>[2x]MPPGKCLFSGVF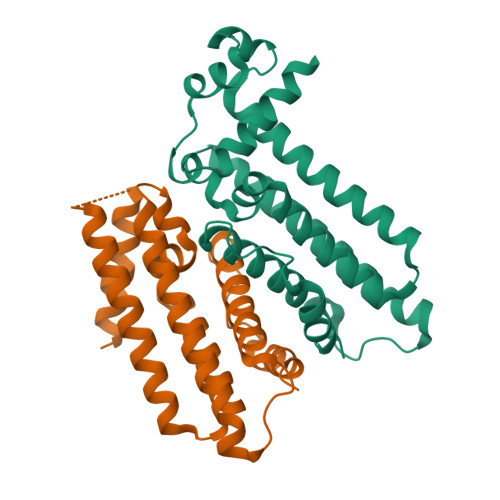CNMAEKQTAKRNRREEILQSLALMLESSDGSQRITTAKLAASVGVSEAALYRHFPSKTRMFDSLIEFIEDSLITRINLILKDEKDTTARLRLIVLLILGFGERNPGLTRILTGHALMFEQDRLQGRINQLFERIEVQLRQVMREKKMREGEGYTLDETLLASQLLAFCEGMLSRFVRSEFKYRPTDDFEARWPLVAAQLQ>[2x]MGLPPLLSLPSNSAPRSLGRVETPPEVVDFMVSLAEAPRGGRVLEPACAHGPFLRAFREAHGTGYRFVGVEID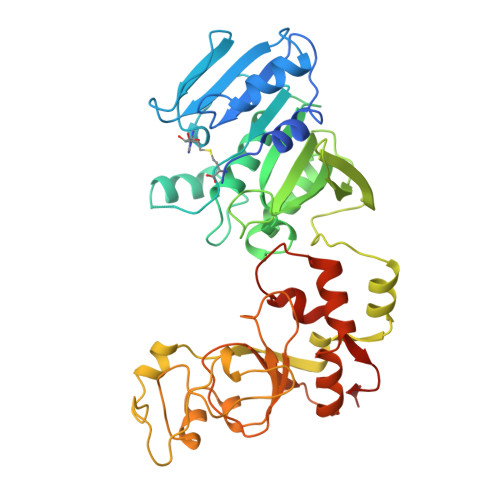PKALDLPPWAEGILADFLLWEPGEAFDLILGNPPYGIVGEASKYPIHVFKAVKDLYKKAFSTWKGKYNLYGAFLEKAVRLLKPGGVLVFVVPATWLVLEDFALLREFLAREGKTSVYYLGEVFPQKKVSAVVIRFQKSGKGLSLWDTQESESGFTPILWAEYPHWEGEIIRFETEETRKLEISGMPLGDLFHIRFAARSPEFKKHPAVRKEPGPGLVPVLTGRNLKPGWVDYEKNHSGLWMPKERAKELRDFYATPHLVVAHTKGTRVVAAWDERAYPWREEFHLLPKEGVRLDPSTLVQWLNSEAMQKHVRTLYRDFVPHLTLRMLERLPVRREYGFHTSPESARNF Creatine is obtained by the diet or synthesized by endogenous enzymes, and specifically transported into the cell using the creatine transporter (CRT), a sodium- and chloride-dependent transporter, belonging to the solute carrier 6 (SLC6) family. Impaired function of CRT leads to intracellular creatine deficiency, resulting in X-linked creatine transporter deficiency (CTD), a disorder characterized by intellectual disability, speech and language delay, behavioral abnormalities, and seizures. The structure of CRT adopts a typical LeuT fold, consisting of 12 transmembrane (TM) helices, with two gating helices, TM1 and TM6, each divided into segments TM1a/1b and TM6a/6b. We determined the cryo-EM structures of CRT in the apo (CRT-apo), and in the presence of substrate creatine (CRT–creatine) or inhibitor RGX (CRT–RGX), at the resolutions of 3.29 Å, 3.40 Å, and 3.39 Å, respectively.

In the structure of CRT-apo, TM1 and TM6 form a translocation pathway accessible exclusively from the cytoplasmic side, suggesting that CRT-apo is in the inward-open state. Notably, in the CRT-apo, a distinct density has been identified as a putative Cl– ion, with no additional densities observed for Na+ ions. In the structure of CRT-apo, TM1a bends ~33° toward the membrane plane, thereby opening the intracellular translocation pathway. Comparison of the inward-open (CRT-apo) and inward-occluded (CRT–creatine and CRT–RGX) structures reveals that the most evident conformational changes are located in TM1a. The conformational changes primarily involved the displacement of TM1a, a phenomenon also observed in GAT1 and GlyT1 during the transition from inward-occluded to inward-open state. Meanwhile, the Cl− ion remains in its conserved position and is not released.

> MAKKSAENGIYSVSGDEKKGPLIAPGPDGAPAKGDGPVGLGTPGGRLAVPPRETWTRQMDFIMSCVGFAVGLGNVWRFPYLCYKNGGGVFLIPYVLIALVGGIPIFFLEISLGQFMKAGSINVWNICPLFKGLGYASMVIVFYCNTYYIMVLAWGFYYLVKSFTTTLPWATCGHTWNTPDCVEIFRHEDCANASLANLTCDQLADRRSPVIEFWENKVLRLSGGLEVPGALNWEVTLCLLACWVLVYFCVWKGVKSTGKIVYFTATFPYVVLVVLLVRGVLLPGALDGIIYYLKPDWSKLGSPQVWIDAGTQIFFSYAIGLGALTALGSYNRFNNNCYKDAIILALINSGTSFFAGFVVFSILGFMAAEQGVHISKVAESGPGLAFIAYPRAVTLMPVAPLWAALFFFMLLLLGLDSQFVGVEGFITGLLDLLPASYYFRFQREISVALCCALCFVIDLSMVTDGGMYVFQLFDYYSASGTTLLWQAFWECVVVAWVYGADRFMDDIACMIGYRPCPWMKWCWSFFTPLVCMGIFIFNVVYYEPLVYNNTYVYPWWGEAMGWAFALSSMLCVPLHLLGCLLRAKGTMAERWQHLTQPIWGLHHLEYRAQDADVRGLTTLTPVSESSKVVVVESVM>GPHMGSRSRLLAANAAAAAFYAQALQSDEAAPARQYLTERSFDAAAARKFGCGFAPSGWDSLTKHLQRKGFEFEELEAAGLSRQGRHGPMDRFHR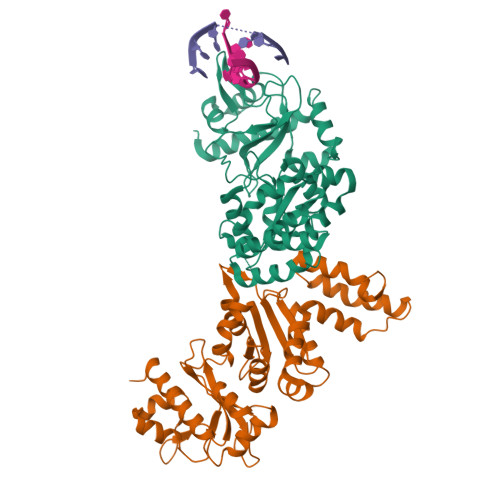RLLWPIRTSAGEVVGFGARRLFDDDAMEAKYVNTPETLLYKKSSVMFGIDLAKRDIAKGHQAVVVEGYTDVMAMHLAGVTTAVASCGTAFGGEHLAMLRRLMMDDSFFRGELIYVFDGDEAGRAAALKAFDGEQKLAGQSFVAVAPDGMDPCDLRLKCGDAALRDLVARRTPLFEFAIRAAIAEMDLDSAEGRVAALRRCVPMVGQIKDPTLRDEYARQLAGWVGWADVA[2x]N-{4-[3-(5-methoxypyridin-2-yl)-1H-pyrrolo[3,2-b]pyridin-2-yl]pyridin-2-yl}acetamide 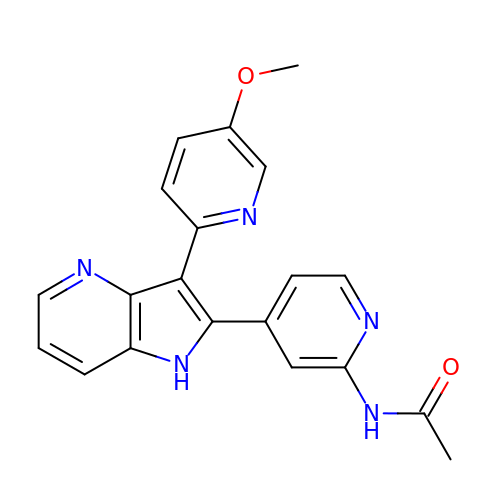| C20 H17 N5 O2 | VRPRBQAJAQCSCW-UHFFFAOYSA-N>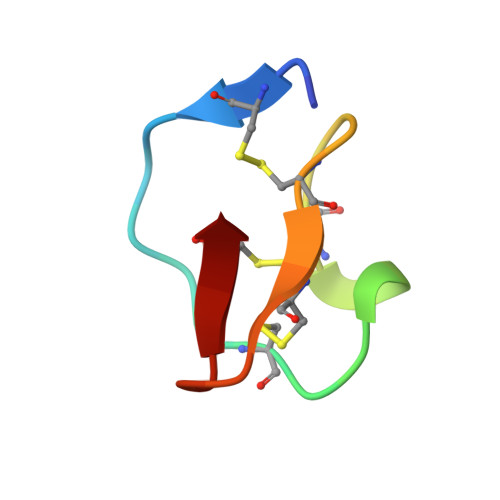 RVCPRILMECKKDSDCLAECVCLEHGYCG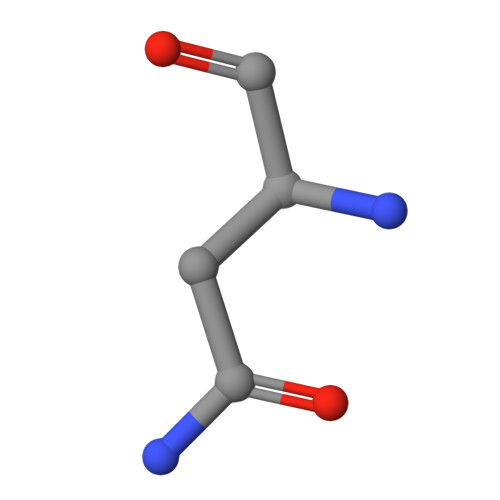> NQ> DEINKELNQVMEQLGDARIDRQESSRQQRKAEIMESIKRLYPGSVYGRLIDLCQPTQKKYQIAVTKVLGKNMDAIIVDSEKTGRDCIQYIKEQRGEPETF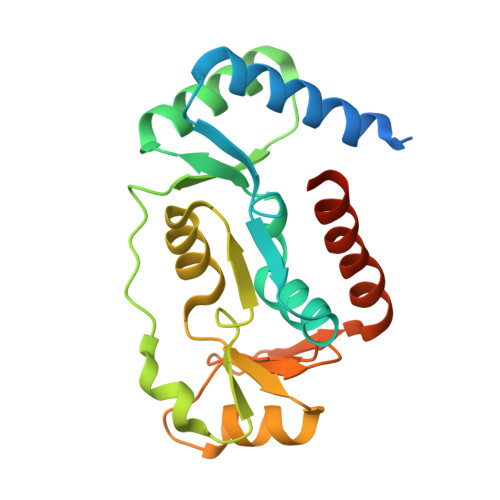LPLYYLEVKPTDEKLRELKGAKLVIDVIRYEPPHIKKALQYACGNALVCDNVEDARRIAFGGHQRHKTVALDGTLFQKSGVISGGASDLKAKARRWDEKAVDKLKEKKERLTEEL>GHMRKYSQRHIPVMVREVIEFLKPEDEKIILDCTVGEGGHSRAILEHCPGCRIIGIDVDSEVLRIAEEKLKEFSDRVSLFKVSYREADFLLKTLGIEKVDGILMDLGVSTYQLKGENRGFTFEREEPLDMRMDLESEVTAQKVLNELPEEELARIIFEYGEEKRFARRIARKIVENRPLNTTLDLVKAVREALPSYEIRRRKRHFATKTFQAIRIYVNRELENLKEFLKKAEDLLNPGGRIVVISFHSLEDRIVKETFRNS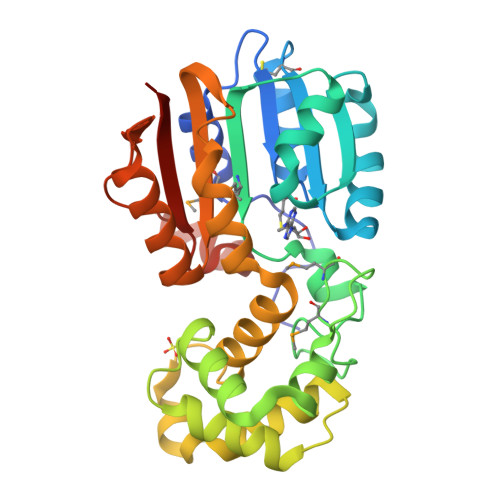KKLRILTEKPVRPSEEEIRENPRARSGRLRAAERIEEGGD[2x]>GGVTDALSLMYSTSTGGPASIAANALTDFDLSGALTVNSVGTGLTKSAAGIQLAAGKSGLYQITMTVKNNTVTTGNYLLRVKYGSSDFVVACPASSLTAGGTISLLIYCNVLGVVSLDVLKFSLCNDGAALSNYI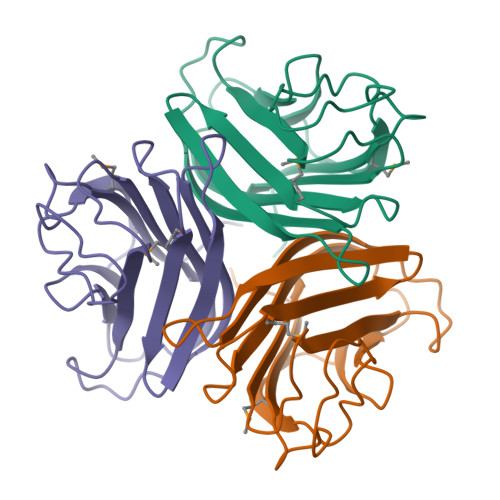INITAAKIN[2x]>MTERIRNVALRSKVCPAETASELIKHGDVVGTSGFTGAGYPKEVPKALAQRMEAAHDRGEKYQISLITGASTGPQLDGELAKANGVYFRSPFNTDATMRNRINAGETEYFDNHLGQVAGRAVQGNYGKFNIALVEATAITEDGGIVPTS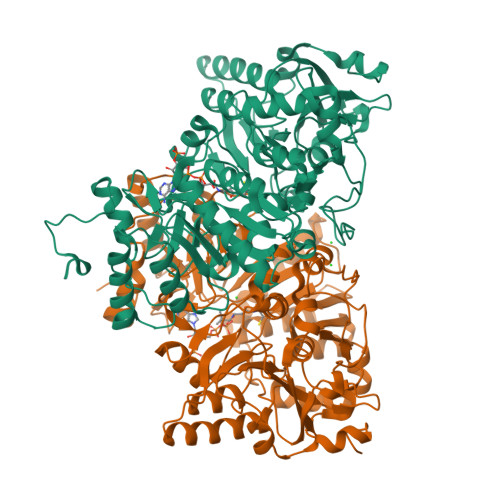SVGNSQTFLNLAEKVIIEVNEWQNPMLEGIHDIWDGNVSGVPTRDIVPIVRADQRVGGPVLRVNPDKIAAIVRTNDRDENAPFAAPDETAKAIAGYLLDFFGHEVKQNRLPPSLLPLQSGVGNVANAVLEGLKEGPFENLVGYSEVIQDGMLAMLDSGRMRIASASSFSLSPEAAEEINNRMDFFRSKIILRQQDVSNSPGIIRRLGCIAMNGMIEADIYGNVNSTRVMGSKMMNGIGGSGDFARSSYLSIFLSPSTAKGGKISAIVPMAAHVDHIMQDAQIFVTEQGLADLRGLSPVQRAREIISKCAHPDYRPMLQDYFDRALKNSFGKHTPHLLTEALSWHQRFIDTGTMLPSSLEHHHHHH[2x]Glucuronyl esterases (GEs) are carbohydrate-active enzymes that are able to cleave ester linkages between the alcohols of the aromatic polymer lignin and 4-O-methylglucuronic acid (4-O-MeGlcA) moieties on glucuronoxylan in the plant cell wall, a linkage which contributes to the recalcitrance of plant biomass. Several more experimental structures have since been obtained, totaling eight structures (three from fungal species and five from bacterial species) from diverse organisms. GEs belong to the α/β hydrolase (ABH) superfamily, with a catalytic triad common to serine hydrolases consisting of a Ser nucleophile, a basic His residue and an acidic Glu/Asp residue. However, one of the putative GEs from Lentithecium fluviatile, LfCE15C, lacks many of the additional sequence characteristics of a fungal CE15-B as described in Ernst et al.. As highlighted in Fig. 1(a), a highly conserved glutamate residue in a substrate-interacting helix-containing loop (here denoted αL) is a glycine in LfCE15C, while a conserved substrate-interacting tryptophan is instead a tyrosine.

The structure was determined to a maximum resolution of 2.65 Å (crystal form A) with good overall geometry. The final model contains four protein chains, each with an N-glycosylation site at Asn241 modelled with variable number of carbohydrate units. As seen in other fungal members of CE15, LfCE15C is stabilized by several disulfide bonds (Cys21–Cys56, Cys199–Cys337 and Cys231–Cys309). The active-site structure is stabilized by one of the disulfide bonds (Cys199–Cys337), also conserved in Cip2, that joins the strand bearing the serine nucleophile to the loop bearing the catalytic histidine. The glutamate residue can presumably be functionally equivalent to glutamine, so this difference is unlikely to be of functional importance. In contrast, the characteristic glutamate of fungal CE15-B further along in the αL region (Glu324 in CuGE), which interacts with O2 of the GlcA moiety as well as the xylan backbone, is substituted by a glycine in LfCE15C (Gly254). Furthermore, an otherwise extremely conserved tryptophan in the whole CE15 family (Trp358 in OtCE15A and Trp368 in CuGE and CE15-B, phenylalanine or tryptophan in fungal CE15-A), which interacts with GlcA O2 and is located at the end of β-strand 7 in the loop following the canonical acid residue position, is found to be a tyrosine in LfCE15C. Although in principle this is a conservative substitution, the hydrogen bond between the NH group of tryptophan and O2 of the GlcA moiety will almost certainly be lost given the conformation of the corresponding tyrosine in the active site.

>[4x]QAPSCPNLPASINYAANPKLPDPFLALSGTRLSKKDQWPCRKEEIRQLFQRYSYGTFPPRPESVTAAMSGNALKITVSEGSKSMSFSVNIKLPSSGAAPYPAIIAYGSASLPIPNTVATITYQNFEMAADNGRGKGKFYEFYGSNHNAGGMIAAAWGVDRIIDALEMTPAAKIDPKRVGVTGCSRNGKGSMIAGAFVDRIALALPQEGGQSAAGCWRIADEIQKNGTKVETAHQIVNGDSWFSTDFSKYVDTVPTLPWDNHMLHALYAYPPRGLLIIENTAIDYLGPTSNYHCATAGRKVHEALGVKDYFGFSQNSHSDHCGFPKAQQPELTAFIERFLLAKDTKTDVWKTDGKFTIDERRWIDWAVPSLSGLEQKLISEEDLNSAVDHHHHHH>[4x]KYELTLQRSLPFIEGMLTNLGAMKLHKIHSFLKITVPKDWGYNRITLQQLEGYLN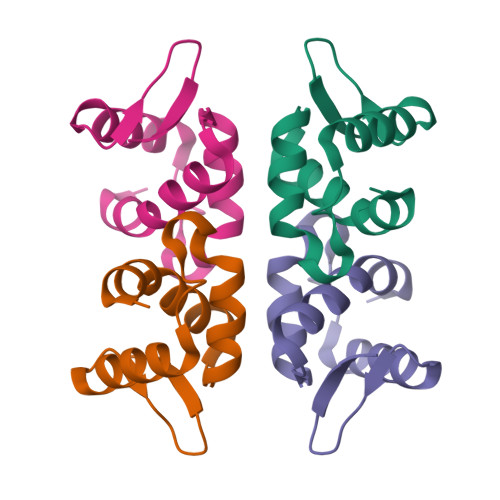TLADEGRLKYIANGSYEIV> GAGSMKSRYTTEFHELEKIGSGEFGSVFKCVKRLDGCIYAIKRSKKPLAGSVDEQNALREVYAHAVLGQHSHVVRYFSAWAEDDHMLIQNEYCNGGSLADAISENYRIMSYFKEAELKDLLLQVGRGLRYIHSMSLVHMDIKPSNIFISRTSIPNAASEEGDEDDWASNKVMFKIGDLGHVTRISSPQVEEGDSRFLANEVLQENYTHLPKA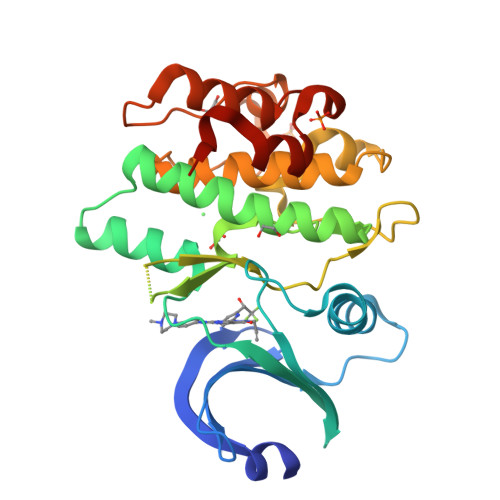DIFALALTVVCAAGAEPLPRNGDQWHEIRQGRLPRIPQVLSQEFTELLKVMIHPDPERRPSAMALVKHSVLLSASRK> MKLQQLRYIVEVVNHNLNVSSTAEGLYTSQPGISKQVRMLEDELGIQIFARSGKHLTQVTPAGQEIIRIAREVLSKVDAIKSVAGEHTWPDKGSLYVATTHTQARYALPGVIKGFIERYPRVSLHMHQGSPTQIAEAVSKGNADFAIATEALHLYDDLVMLPCYHWNRSIVVTPEHPLATKGSVSIEELAQYPLVTYTFGFTGRSELDTAFNRAGLTPRIVFTATDADVIKTYVRLGLGVGVIASMAVDPVSDPDLVKLDANGIFSHSTTKIGFRRSTFLRSYMYDFIQRF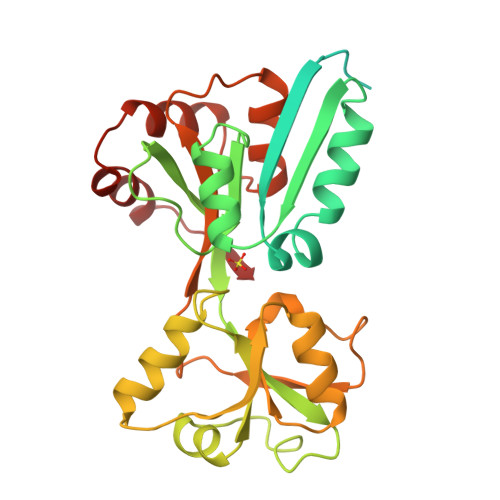APHLTRDVVDTAVALRSNEDIEAMFKDIKLPEK>SVLVLDDRIVDAATKDLYVNGFQEEIQYQNPTPENLQHMFHQGIEILDSARMINVTHLALWKPSSFKLGNPVDFALDDNYDTFWQSDGGQPHQLDIMFSKRMDICVMAIFFSMIADESYAPSLVKVYAGHSPSDARFYKMLEVRNVNGWVALRFLDNREDDQLLKCQFIRLLFPVNHENGKDTHLRGIRLYVPSNEPHQDTHE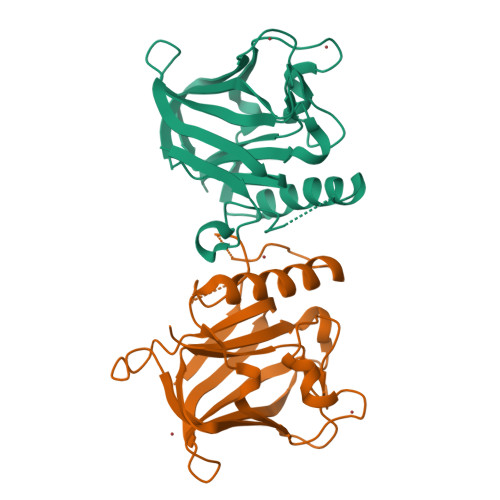WAQTLPETNNVFQDAILR[2x]>MA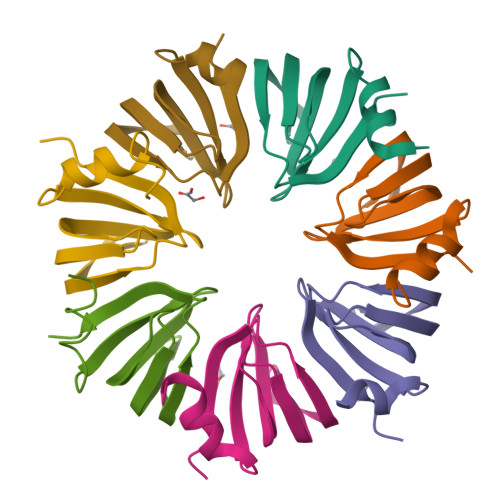SDISKCFATLGATLQDSIGKQVLVKLRDSHEIRGILRSFDQHVNLLLEDAEEIIDGNVYKRGTMVVRGENVLFISPVPG[7x]(4-{7-[2-(4-chlorophenoxy)ethyl]-2-(methylamino)-6-oxo-6,7-dihydro-1H-purin-8-yl}phenyl)phosphonic acid | C20 H19 Cl N5 O5 P | 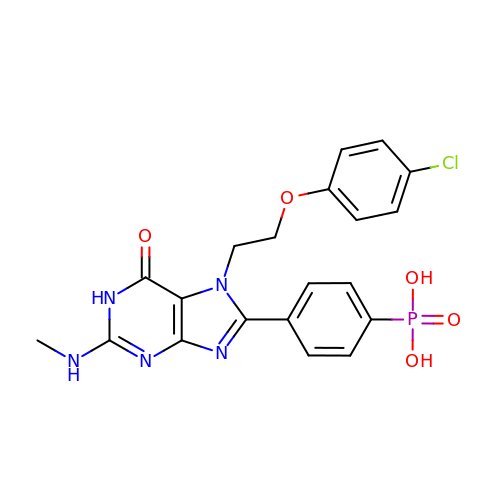MCYZBWKMUOPJOU-UHFFFAOYSA-N methyl (2~{S})-2-[[(2~{R},4~{a}~{S},6~{a}~{R},6~{a}~{S},14~{a}~{S},14~{b}~{R})-2,4~{a},6~{a},6~{a},9,14~{a}-hexamethyl-10-oxidanyl-11-oxidanylidene-1,3,4,5,6,13,14,14~{b}-octahydropicen-2-yl]carbamoylamino]-3-oxidanyl-propanoate 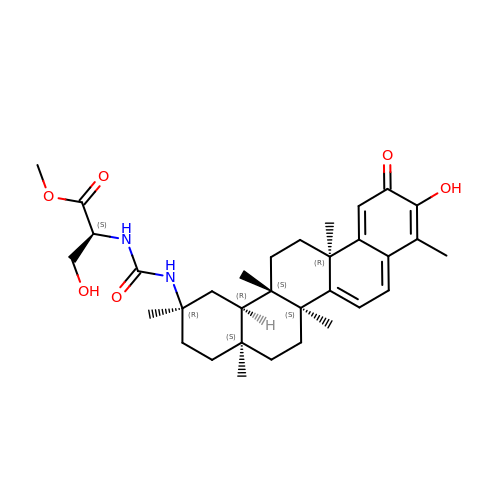| C33 H46 N2 O6 | PJLZTFVARNCYGK-CPKSEDGTSA-N>GHHHHHHG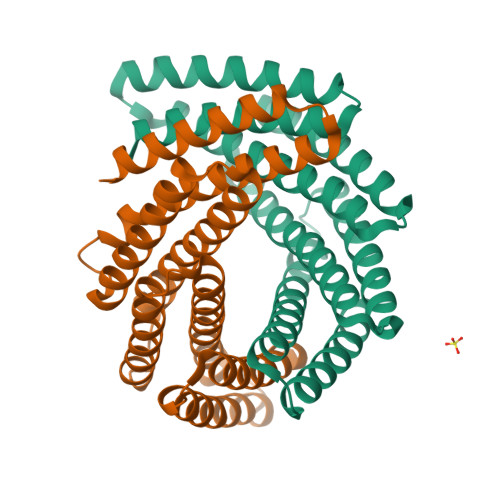SGSGENLYFQSGSGSSPELDELWKRVKKLVTELLEQAERAGDPEEIFKLLEVAAALVFLAEMFLRLAAIQEKATDPEIQELAERVLRLIKRLLEEAERAGDPRRIRELVEVASQLAFLLELFYRLKEIQERATDPEIQELAERVLRLIKKLLKAAEEAGDPRKIHKLVFVAIVLLFLLQTFYRLKEIQEKATDPEIQRKAQEVLEKIKRLLEAAERAGDPAKILLYVIRALLLAMELKFAYRKR[2x]>[2x]SNSASSCHRPLLIPPVRPVGPGRA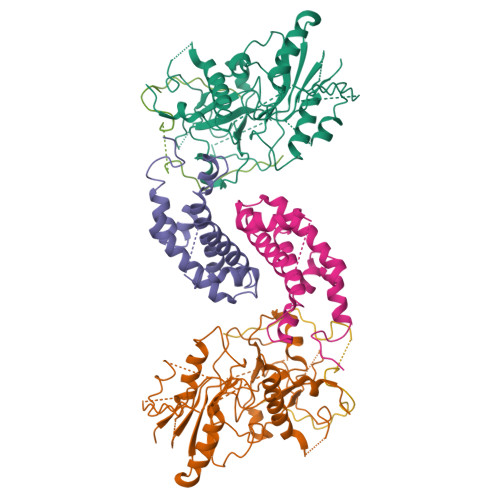LLLLPVEQGFTFSGICRVTCLYGQVQVFGFTISQGQPAQDIFSVYTHSCLSIHALHYSQPEKSKKELKREARNLLKSHLNLDDRRWSMQNFSPQCSIVLLEHLKTATVNFITSYPGSSYIFVQESPTPQIKPEYLALRSVGIRREKKRKGLQLTESTLSALEELVNVSCEEVDGCPVILVCGSQDVGKSTFNRYLINHLLNSLPCVDYLECDLGQTEFTPPGCISLLNITEPVLGPPFTHLRTPQKMVYYGKPSCKNNYENYIDIVKYVFSAYKRESPLIVNTMGWVSDQGLLLLIDLIRLLSPSHVVQFRSDHSKYMPDLTPQYVDDMDGLYTKSKTKMRNRRFRLAAFADALEFADEEKESPVEFTGHKLIGVYTDFAFRITPRNRESHNKILRDLSILSYLSQLQPPMPKPLSPLHSLTPYQVPFNAVALRITHSDVAPTHILYAVNASWVGLCKIQDDVRGYTNGPILLAQTPICDCLGFGICRGIDMEKRLYHILTPVPPEELRTVNCLLVGAIAIPHCVLKCQRGIEGTVPYVTTDYNFKLPGASEKIGAREPEEAHKEKPYRRPKFCRKMK;>SNMSWESGAGPGLGSQGMDLVWSAWYGKCVKGKGSLPLSAHGIVVAWLSRAEWDQVTVYLFCDDHKLQRYALNRITVWRSRSGNELPLAVASTADLIRCKLLDVTGGLGTDELRLLYGMALVRFVNLISERKTKFAKVPLKCLAQEVNIPDWIVDLRHELTHKKMPHINDCRRGCYFVLDWLQKTYWCRQLENSLRETWELE[2x];>SNGQESPTAENARLLAQKRGALQGSAWQVSSEDVRWDTFPLGRMPGQTEDPAELMLENYDTMYLLDQPVLE[2x]CDC7 is an essential Ser/Thr kinase that acts upon the replicative helicase throughout the S phase of the cell cycle and is activated by DBF4. CDC7 possesses the canonical bilobal kinase fold, which is interrupted by unique kinase inserts (KIs). The structures reveal a zinc-finger domain at the end of the kinase insert 2 that pins the CDC7 activation loop to motif M of DBF4 and the C lobe of CDC7. We conclude that CDC7 activity is controlled by DBF4 at two levels: (1) via ordering of the activation loop dependent on the ZF domain-DBF4 motif M interactions; and (2) via the control of αC insertion through by DBF4 motif C (Hughes et al., 2012).

Co-crystallization was only successful using the bisubstrate approach with MCM2(33–47) peptide covalently conjugated to ATPγS via bromoacetyl-aminoalanine in place of Ser40 and pre-phosphorylated on Ser41. X-ray diffraction data were collected to 1.7-Å resolution, and the structure was solved by molecular replacement. The nucleotide bound in the active site and nine residues of the substrate peptide, spanning MCM2 residues 38–46, were built in the resulting electron density map. No density could be attributed to the γ-phosphate moiety, presumably due to hydrolysis of the bisubstrate ligand during crystallization. In the crystal structure, the phosphate group on Ser41 of the target peptide, mimicking priming by CDK2, forms well-defined interactions with side chains of Arg373 and Arg380, invariant residues from the CDC7 activation loop and the C lobe, respectively. Accordingly, substitution of either or both of these residues to Ala compromised the kinase activity. In addition to the interactions involving MCM2 phospho-Ser41, the side chain of Arg44, located in P+4 substrate position, is buried in a pocket lined by CDC7 and DBF4 residues. Within the pocket, MCM2 Arg44 makes a salt bridge with DBF4 Glu297 and hydrogen bonds with Ser96 and Gly198 of CDC7, stacking against CDC7 Phe96. Concordantly, substitutions of Arg44 in the context of the substrate peptide resulted in relatively minor defects of the in vitro kinase activity, in sharp contrast to the near complete loss of phosphorylation upon removal of the priming phosphate on Ser41. The ordering of the activation loop allowed co-crystallization of the kinase in complex with a target peptide.

> LAGVKKDIEKLYEAVPQLSNVFKIEDKIGEGTFSSVYLATAQLQVGPEEKIALKHLIPTSHPIRIAAELQCLTVAGGQDNVMGVKYCFRKNDHVVIAMPYLEHESFLDILNSLSFQEVREYMLNLFKALKRIHQFGIVHRDVKPSNFLYNRRLKKYALVDFGLAQGTHDTKIELLKFVQSEAQQERCSQNKPASLTCDCYATDKVCSICLSRRQQVAPRAGTPGFRAPEVLTKCPNQTTAIDMWSAGVIFLSLLSGRYPFYKASDDLTALAQIMTIRGSRETIQAAKTFGKSILCSKEVPAQDLRKLCERLRGAGAGGWNEVPDEAYDLLDKLLDLNPASRITAEEALLHPFFKDMSL;> GPGTRTGRLKKPFVKVEDMSQLYRPFYLQLTNMPFINYSIQKPCSPFDVDKPSSMQKQTQVKLRIQTDGDKYGGTSIQLQLKEKKKKGYCECCLQKYEDLETHLLSEQHRNFAQSNQYQVVDDIVSKLVFDFVEYEKDTPKKKR;> RRTDALTASPGRDLP>[2x]NGNSLSAAELTCGMIMCLARQIPQATASMKDGKWERKKFMGTELNGKTLGILGLGRIGREVATRMQSFGMKTIGYDPIISPEVSASFGVQQLPLEEIWPLCDFITVHTPLLPSTTGLLNDNTFAQCKKGVRVVNCARGGIVDEGALLRALQSGQCAGAALDVFTEEPPRDRALVDHENVISCPHLGASTKEAQSR

Human 3-phosphoglycerate dehydrogenase (PHGDH) is responsible for the NAD+-dependent conversion of 3-phosphoglycerate (3-PG) to phosphohydroxypyruvate (PHP), which is the first step in the de novo serine synthesis pathway. Thus, PHGDH activity diverts glycolytic flux into biomass production. Limited proteolysis with thermolysin revealed a stable fragment of PHGDH consisting of the core of the catalytic domain containing the cofactor-binding site, and this was shown to crystallise readily. Thus PHGDH-93 provides a valuable tool to investigate binders to the cofactor-binding site.

PHGDH-93 was then successfully crystallised with an empty, accessible cofactor-binding pocket. Soaking of all 15 fragments into PHGDH-93 crystals was performed overnight at RT using a fragment concentration of 80 mM in 20 % DMSO. All of the fragments for which crystallographic data were obtained bound to the adenine-pocket suggesting this pocket to be a preferential site for fragment binding. Analysis of the fragments’ binding modes showed that four of the fragments (5, 14, 15 and 16) were coordinated by hydrogen and/or halogen bonds, whereas the other three fragments (3, 9 and 10) appeared to be stabilised only by apolar contacts. Of the four compounds forming specific interactions with the protein, fragments 5 (3-chloro-4-fluorobenzamide), 14 (5-fluoro-2-methylbenzoic acid) and 15 (N-(3-chloro-4-methoxyphenyl)acetamide) constitute substituted benzene rings. The most potent compound according to the ITC data, fragment 5, bound more deeply in the adenine binding pocket compared to the other two structurally similar fragments, and formed an halogen bond with the backbone carbonyl of Gly151 through its chloro atom and a hydrogen bond with the side-chain of Ser211. Fragment 15 formed a similar halogen bond interaction with Gly151 through a chloro-substituent. Fragment 14 was substantially less potent (Kd = 26 ± 31 mM) compared to the two structurally similar fragments 5 and 15 (5, Kd = 1.6 ± 0.2 mM and 15, Kd = 2.8 ± 1.6 mM).5-[1-[(1~{R})-1-[5-[3-chloranyl-2-fluoranyl-6-(1,2,3,4-tetrazol-1-yl)phenyl]-1-oxidanyl-pyridin-2-yl]-2-cyclopropyl-ethyl]pyrazol-4-yl]-6-methyl-pyridin-2-amine 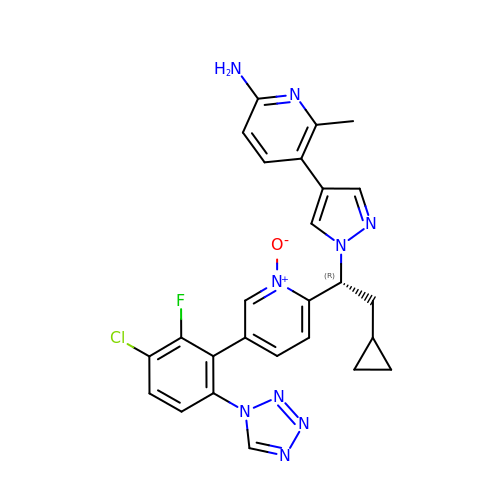| C26 H23 Cl F N9 O | LGWUJLNQWXJMJR-HSZRJFAPSA-N> GPEVQKPLHEQLWYHGAIPRAEVAELLVHSGDFLVRESQGKQEYVLSVLWDGLPRHFIIQSLDNLYRLEGEGFPSIPLLIDHLLSTQQPLTKKSGVVLHRAVPKDKWVLNHEDLVLGEQIGRGNFGEVFSGRLRADNTLVAVKSCRETLPPDLKAKFLQEARILKQYSHPNIVRLIGVCTQKQPIYIVMELVQGGDFLTFLRTEGARLRVKTLLQMVGDAAAG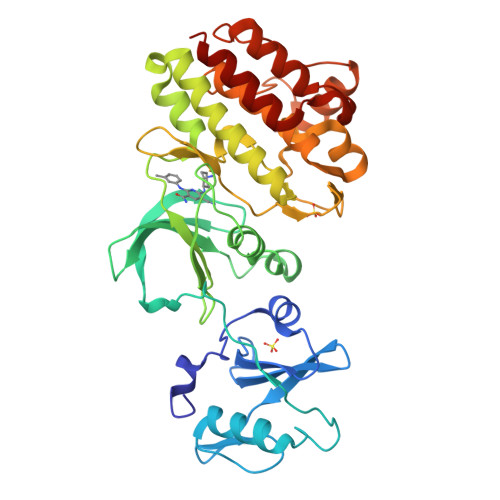MEYLESKCCIHRDLAARNCLVTEKNVLKISDFGMSREEADGVYAASGGLRQVPVKWTAPEALNYGRYSSESDVWSFGILLWETFSLGASPYPNLSNQQTREFVEKGGRLPCPELCPDAVFRLMEQCWAYEPGQRPSFSTIYQELQSIRKRHR> APTNEFY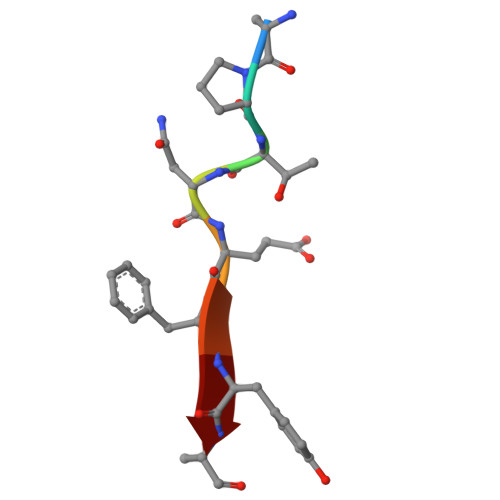A>MGSSHHHHHHSQDPNSSSMAASEGVLLGMGNPLLDISAVVDDAFLTKYDIKLNNAILAEEKHLPMYDELASKSNVEYIAGGATQNSIRVAQWMLQTPGATSYMGCIGKDKFGEEMKKNAQAAGVTAHYYEDETAPTGTCAVCVVGGERSLIANLSAANCYKSEHLKRPENWALVEKAKYIYIAGFFLTVSPDSIQLVAEHAAANNKVFLMNLSAPFICEFFRDAQEKVLPYADYIFGNETEAKIFAKVRGWETENIEEIALKISQLPLASGKQKRIAVITQGADPVVVAEDGKVKTFPVILLPKEKLVDTNGAGDAFVGGFLSQLVLGKGIEDCVRAGCYAANVIIQRPGCTYPEKPDFN[2x]

Adenosine undergoes ATP-dependent phosphorylation catalyzed by adenosine kinase (ADK). In plants, ADK also phosphorylates cytokinin ribosides, transport forms of the hormone. We discovered that maize and moss enzymes can form dimers upon increasing protein concentration, setting them apart from the monomeric human and protozoal ADKs. Structural and kinetic analyses revealed a catalytically inactive unique dimer.

Of the two selected representatives, ZmADK2 and PpADK1, we only obtained crystals of the apo form of ZmADK2. Crystallization conditions of ZmADK2 favored the dimeric form to be present in the asymmetric unit, which contains two ZmADK2 molecules, each in the open conformation, and resembles that of HsADK, with an average root mean square deviation (RMSD) of ~1.2 Å and 1.4 Å for all Cα atoms. Each monomer is composed of two domains: a large 10-stranded α/β Rossmann-like nucleotide-binding domain (residues 1–14, 64–117, and 137–340) comprising the ATP-binding site; and a small five-stranded α/β domain (residues 17–61 and 120–134). The small domain encompases β2, β3, β4, β8, and β9 sheets, plus α1 and α2 helices. Both domains are connected via four peptide hinges (Leu15–Leu16, Gly62–Gly63, Thr118–Gly119, and Asn135–Leu136). The existence of the dimer was further confirmed by X-ray crystallography on ZmADK2, and the structure explains why this oligomeric state is not functional. So far, such a dimer arrangement has not been reported for any other ADK. Remarkably, the dimer interface prevents displacement of the small domains. We further showed that the ADK dimer can exist only when both subunits are in an open conformation, as observed in the ZmADK2 structure. When in a dimeric state, the enzyme cannot be catalytically active as the rotation of the small domain and closure of the substrate cavity for catalysis is blocked. Therefore, to be active, moss and maize ADK dimers must be dissociated into monomers.(3~{S})-3-(phenylsulfonylmethyl)piperidine-2,6-dione | C12 H13 N 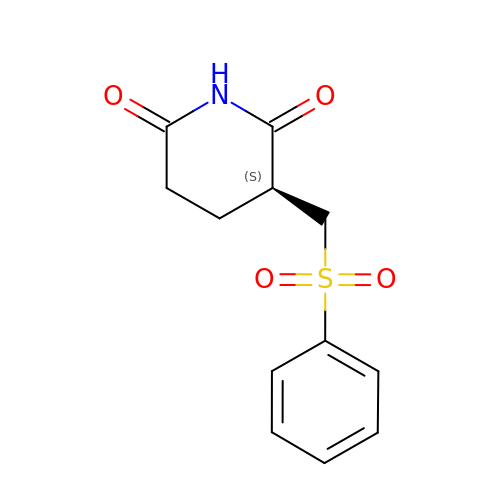O4 S | JPOLQZHTTNLNIA-SECBINFHSA-N> MASSINPWILTGFADAEGSFLLRIRKNNKSSVGYSTELGFQITLHNKDKSILENIQSTWGVGVIANSGDNAVSLKVTRFEDLKVIIDHFEKYPLITQKYADYMLFKQAFNVMENKEHLTIEGIKELVRIKAKLNWGLTDELKKAFPEIISKERSLINKNIPNFKWLAGFTSGDGCFFVNLSKKKTKLGVQVKL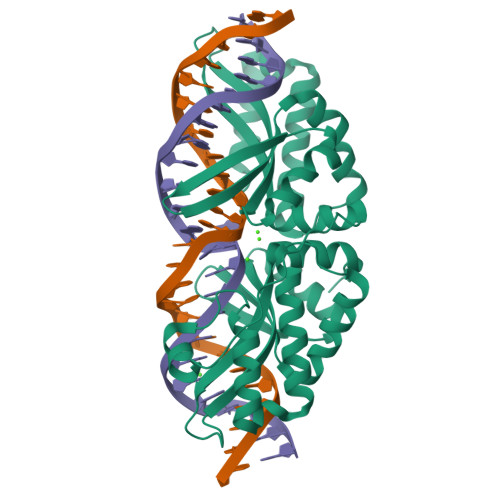VFSISQHIRDKNLMNSLITYLGCGYIKKKNKSEFSWLEFVVTKFSDIRDKIIPFFQEYTLIGTKLKDFEDWCKVAKLIEEKKHLTEEGLDEIKKIKLNMNKGR> PNVSRTIARELKSFLLEYTDETGRSVYGARIRTLGEMNSESLEVNYRHLAESKAILALFLAKCPEEMLKIFDLVAMEATELHYPDYARIHSEIHVRISDFPTIYSLRELRESNLSSLVRVTGVVTRRTGVFPQLKYVKFNCLKCGSILGPFFQDSNEEIRISFCTNCKSKGPFRVNGEKTVYRNYQRVTLQEAPGTVPPGRLPRHREVILLADLVDVSKPGEEVEVTGIYKNNYDGNLNAKNGFPVFATIIEANSIKRREGNTANEGEEGLDVFSWTEEEEREFRKISRDRGIIDKIISSMAPSIYGHRDIKTAVACSLFGGVPKNVNGKHSIRGDINVLLLGDPGTAKSQILKYVEKTAHRAVFATGQGASAVGLTASVRKDPITKEWTLEGGALVLADKGVCLIDEFDKMNDQDRTSIHEAMEQQSISISKAGIVTTLQARCSIIAAANPNGGRYNSTLPLAQNVS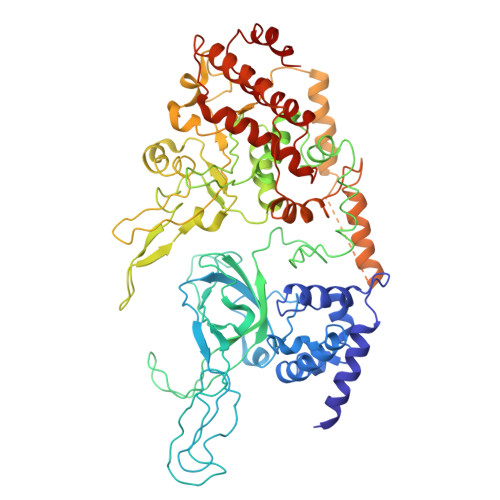LTEPILSRFDILCVVRDLVDEEADERLATFVVDSHVRSHPENDEDREGEELKNNGESAIEQGEDEINEQLNARQRRLQRQRKKEEEISPIPQELLMKYIHYARTKIYPKLHQMDMDKVSRVYADLRRESISTGSFPITVRHLESILRIAESFAKMRLSEFVSSYDLDRAIKVVVDSFVDAQKVSVRRQLRRSFAIY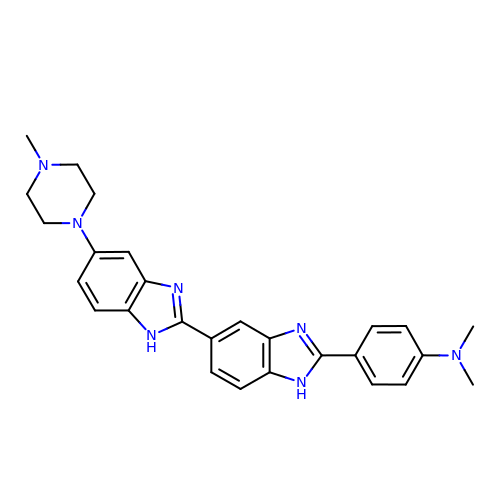2'-(4-DIMETHYLAMINOPHENYL)-5-(4-METHYL-1-PIPERAZINYL)-2,5'-BI-BENZIMIDAZOLE | C27 H29 N7 | VMCOQLKKSNQANE-UHFFFAOYSA-N>MPMQMFMQVYDEIQMFLLEELELKFDMDPNRVRYLRKMMDTTCLGGKYNRGLTVIDVAESLLSLSPNNNGEEDDGARRKRVLHDACVCGWMIEFLQAHYLVEDDIMDNSVTRRGKPCWYRHPDVTVQCAINDGLLLKSWTHMMAMHFFADRPFLQDLLCRFNRVDYTTAVGQLYDVTSMFDSNKLDPDVSQPTTTDFAEFTLSNYKRIVKYKTAYYTYLLPLVMGLIVSEALPTVDMGVTEELAMLMGEYFQV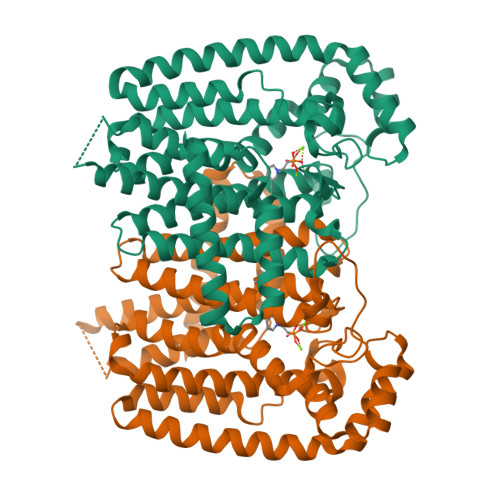QDDVMDCFTPPERLGKVGTDIQDAKCSWLAVTFLAKASSAQVAEFKANYGSGDSEKVATVRRLYEEADLQGDYVAYEAAVAEQVKELIEKLRLCSPGFAASVETLWGKTYKRQK[2x]> GEFGSPSPEEAQLWSEAFDELLASKYGLAAFRAFLKSEFCEENIEFWLACEDFKKT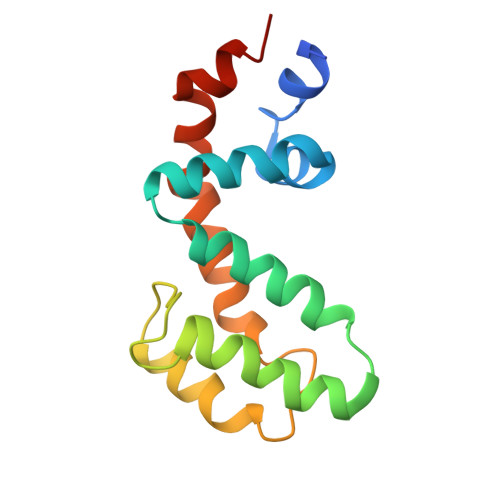KSPQKLSSKARKIYTDFIEKEAPKEINIDFQTKTLIAQNIQEATSGCFTTAQKRVYSLMENNSYPRFLESEFYQDLCKKPQ>AHMSTGEAIPRVAVVVFILNGNSILLGR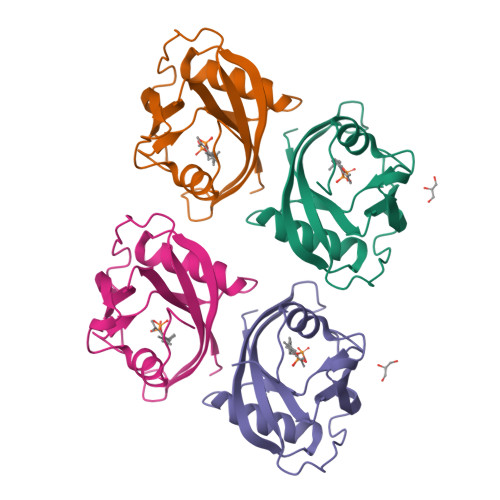RRSSIGNSTFALPGGHLEFGESFEECAAREVMEETGLKIEKMKLLTVTNNVFKEAPTPSHYVSVSIRAVLVDPSQEPKNMEPEKCEGWDWYDWENLPKPLFWPLEKLFGSGFNPFTHGGGD[4x]>GSHMASPNGQTKPLPALKLALEYIVPAMNKHGICVVDDFLGKETGQQIGDEVRALHDTGKFTDGQLVSQKSDSSKDIRGDKITWIEGKEPGCETIGLLMSSMDDLICHCNGKLGSYKINGRTKAMVACYPGNGTGYVRHCDNPNGDGRCVTCIYYLNKDWDAKVSGGILRIFPEGKAQFADIEPKFDRLLFFWSDRRNPHEVQPAYATRYAITVWYFDADERAAAKVKYLTGEKGVRVELNKPSDSVGKDVF[2x];>DACTLLAPAAGDTIISLCF[2x]

The ferrous iron and 2-oxoglutarate (2OG)-dependent HIF prolyl hydroxylases (PHDs/EGLNs) catalyse trans-4-prolyl hydroxylations on HIFα subunits, thus promoting their binding to the von Hippel–Lindau protein (VHL), a targeting component of a ubiquitin E3 ligase, and signalling for HIFα degradation under normoxic conditions. The PHD-catalysed hydroxylations of HIF-1α/HIF-2α in higher animals occur in amino- and carboxy-terminal oxygen-dependent degradation domains (NODD and CODD). The three human PHDs exhibit different NODD/CODD selectivities, with PHD3 being substantially more selective for CODD than PHD1/2 (refs 16). Biophysical analyses employing crystallography and NMR reveal that the molecular basis of PHD isoform and variant selectivity involves enzyme–substrate interactions involving β2/β3 loop residues (that bind the LXXLAP motif) and helices α3 and α4, regions which display sequence variations between the PHD isoforms.

We then used a ‘disulfide cross-linking' strategy to form stable PHD2.Mn.NOG.NODD complexes, where PHD2QM1 (C201A/P317C/R281C/R398A) or PHD2QM2 (C201A/V314C/R281C/R398A) and NODDDC (L397C/D412C) are cross-linked via appropriately positioned cysteines. Binding of ODD residues C-terminal of the target prolines involves DSBH βVIII, βIII, helix α3 and the α3-βI loop. NODD makes more hydrophobic contacts than CODD with the C-terminal region of PHD2.> THETGTTNTATTATS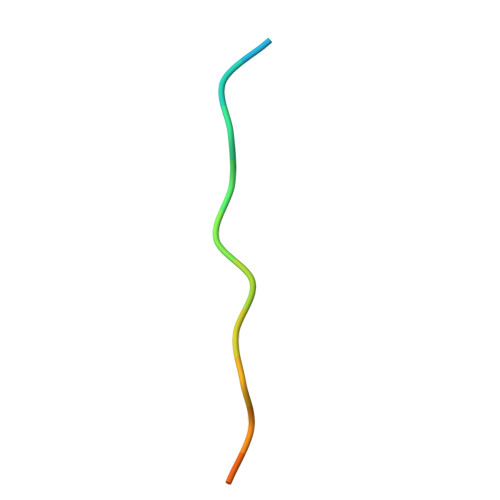N>[2x]GMKDNYDAPESMLTGRVMYNGEALQLRGNEAVQLQLYQHGYAKHDPINVYVNQDGMYSANLFDGEYQMITKSGNGPWTSEGRDTINVTVAGNTVQDVEVTPYYLVRDAQMT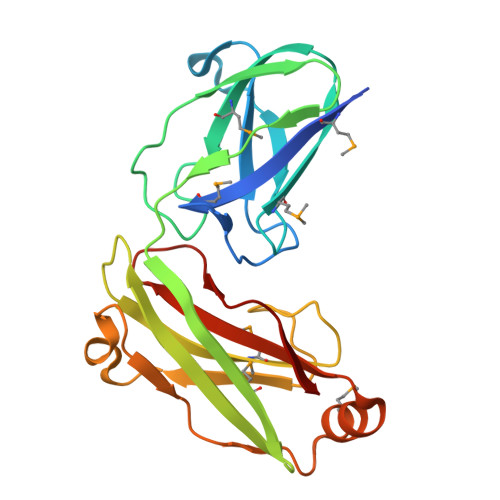LEGNKVNASFKVEKVAGGGIDRVFFMLSTTQFVNDAEHNVDRYDETDNLDAYDETGKLYTFATRDYTDNSMFQTALKRGTLFGRICIWPKGSDQGIYSKVIRLK> GLECKPRPLHKTCSLFMRNIAPNIS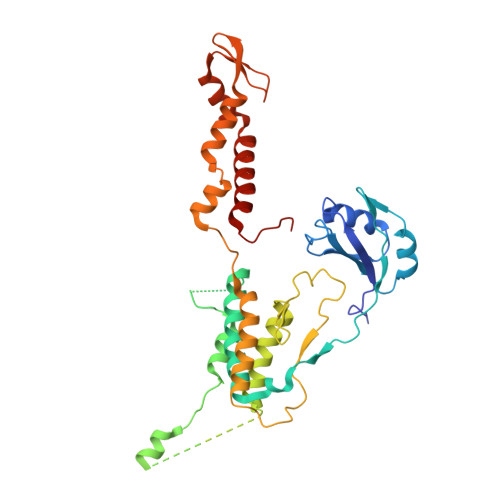RAEIISLCKRYPGFMRVALSEPQPERRFFRRGWVTFDRSVNIKEICWNLQNIRLRECELSPGVNRDLTRRVRNINGITQHKQIVRNDIKLAAKLIHTLDDRTQLWASEPGTPPLPTSLPSQNPILKNITDYLIEEVSAEEEELLGSSGGAPPEEPPKEGNPAEINVERDEKLIKVLDKLLLYLRIVHSLDYYNTCEYPNEDEMPNRCGIIHVRGPMPPNRISHGEVLEWQKTFEEKLTPLLSVRESLSEEEAQKMGRKDPEQEVEKFVTSNTQELGKDKWLCPLSGKKFKGPEFVRKHIFNKHAEKIEEVKKEVAFFNNFLTDAKRPALPE>[2x]IVPTRELENVFLGRCKDYEITRYLDILPRVRSDCSALWKDFFKAFSFKNPCDLDLGSYKDFFTSAQQQLPKNKVMFWSGVYDEAHDYANTGRKYITLEDTLPGYMLNSLVWCGQRANPGFNEKVCPDFKTCPVQARESFWGMASSSYAHSAEGEVTYMVDGSNPKVPAYRPDSFFGKYGLPNLTNKVTRVKVIVLHRLGEKIIEKCGAGSLLDLEKLVKAKHFAFDCVENPRAVLFLLCSD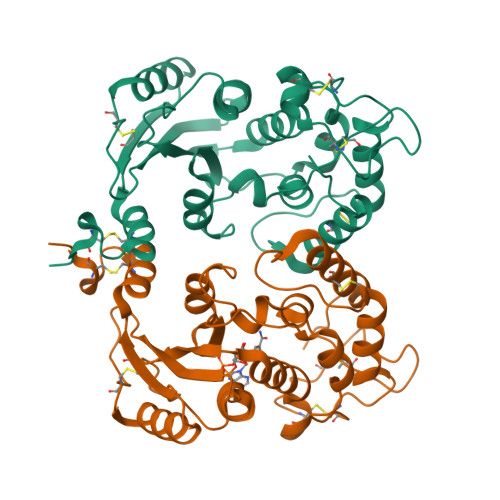NPNARECRLAKRFYRIA> EDGGS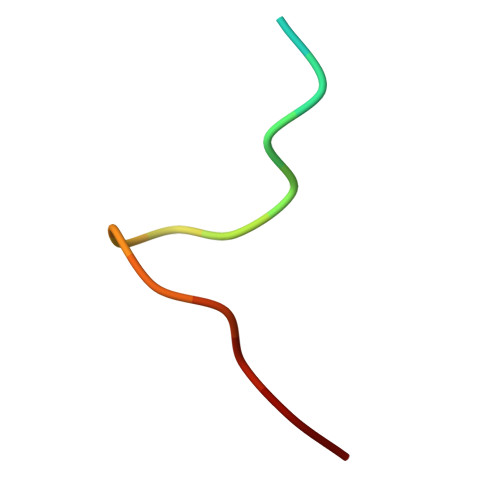WKYPDAFELSG>MVPISPIETVPVKLKPGMDGPKVKQWPLTEEKIKALVEICTEMEKEGKISKIGPENPYNTPVFAIKKKDSTKWRKLVDFRELNKRTQDFWEVQLGIPHPAGLKKKKSVTVLDVGDAYFSVPLDEDFRKYTAFTIPSINNETPGIRYQYNVLPMGWKGSPAIFQSSMTKILEPFKKQNPDIVIYQYMDDLYVGSDLEIGQHRTKIEELRQHLLRWGLTTPDKKHQKEPPFLWMGYELHPDKWTVQPIVLPEKDSWTVNDICKLVGKLNWASQIYPGIKVRQLSKLLRGTKALTEVIPLTEEAELELAENREILKEPVHGVYYDPSKDLIAEIQKQGQGQWTYQIYQEPFKNLKTGKYARMRGAHTNDVKQLTEAVQKITTESIVIWGKTPKFKLPIQKETWETWWTEYWQATWIPEWEFVNTPPLVKLWYQLEKEPIVGAETFYVDGAANRETKLGKAGYVTNKGRQKVVPLTNTTNQKTELQAIYLALQDSGLEVNIVTNSQYALGIIQAQPDKSESELVNQIIEQLIKKEKVYLAWVPAHKGIGGNEQVDKLVSA[2x];>PISPIETVPVKLKPGMDGPKVKQWPLTEEKIKALVEICTEMEKEGKISKIGPENPYNTPVFAIKKKDSTKWRKLVDFRELNKRTQDFWEVQLGIPHPAGLKKKKSVTVLDVGDAYFSVPLDEDFRKYTAFTIPSINNETPGIRYQYNVLPQGWKGSPAIFQSSMTKILEP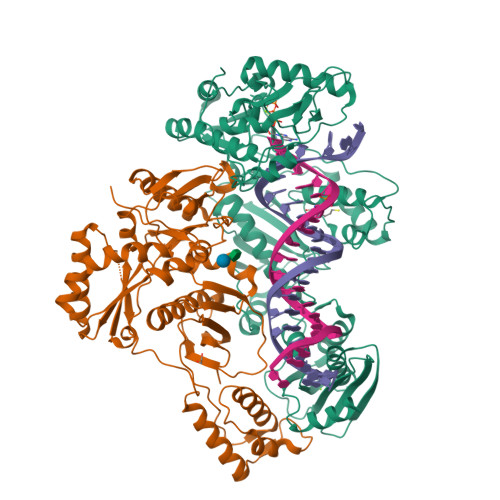FKKQNPDIVIYQYMDDLYVGSDLEIGQHRTKIEELRQHLLRWGLTTPDKKHQKEPPFLWMGYELHPDKWTVQPIVLPEKDSWTVNDIQKLVGKLNWASQIYPGIKVRQLSKLLRGTKALTEVIPLTEEAELELAENREILKEPVHGVYYDPSKDLIAEIQKQGQGQWTYQIYQEPFKNLKTGKYARMRGAHTNDVKQLTEAVQKITTESIVIWGKTPKFKLPIQKETWETWWTEYWQATWIPEWEFVNTPPLVKLWYQ[2x]> MATQHTQYPDARLSSPIVLDQCDLVTRACGLYSSYSLNPQLRNCKLPKHIYRLKYDVTVTKFLSDVPVATLPIDFIVPILLKALSGNGFCPVEPRCQQFLDEIIKYTMQDALFLKYYLKNVGAQEDCVDDHFQEKILSSIQGNEFLHQMFFWYDLAILTRRGRLNRGNSRSTWFVHDDLIDILGYGDYVFWKIPISLLPLNTQGIPHAAMDWYQTSVFKEAVQGHTHIVSVSTADVLIMCKDLITCRFNTTLISKIAEVEDPVCSDYPNFKIVSMLYQSGDYLLSILGSDGYKIIKFLEPLCLAKIQLCSKYTERKGRFLTQMHLAVNHTLEEITEIRALKPSQAHKIREFHRTLIRLEMTPQQLCELFSIQKHWGHPVLHSETAIQKVKKHATVLKALRPIVIFETYCVFKYSIAKHYFDSQGSWYSVTSDRNLTPGLNSYIKRNQFPPLPMIKELLWEFYHLDHPPLFSTKIISDLSIFIKDRATAVERTCWDAVFEPNVLGYNPPHKFSTKRVPEQFLEQENFSIENVLSYAQKLEYLLPQYRNFSFSLKEKELNVGRTFGKLPYPTRNVQTLCEALLADGLAKAFPSNMMVVTEREQKESLLHQASWHHTSDDFGEHATVRGSSFVTDLEKYNLAFRYEFTAPFIEYCNRCYGVKNVFNWMHYTIPQCYMHVSDYYNPPHNLTLENRNNPPEGPSSYRGHMGGIEGLQQKLWTSISCAQISLVEIKTGFKLRSAVMGDNQCITVLSVFPLETDADEQEQSAEDNAARVAASLAKVTSACGIFLKPDETFVHSGFIYFGKKQYLNGVQLPQSLKTATRMAPLSDAIFDDLQGTLASIGTAFERSISETRHIFPCRIT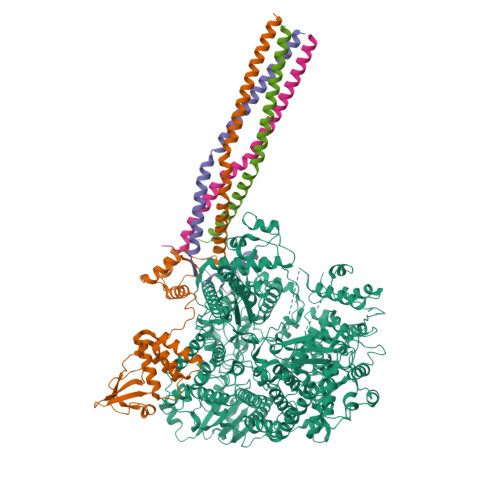AAFHTFFSVRILQYHHLGFNKGFDLGQLTLGKPLDFGTISLALAVPQVLGGLSFLNPEKCFYRNLGDPVTSGLFQLKTYLRMIEMDDLFLPLIAKNPGNCTAIDFVLNPSGLNVPGSQDLTSFLRQIVRRTITLSAKNKLINTLFHASADFEDEMVCKWLLSSTPVMSRFAADIFSRTPSGKRLQILGYLEGTRTLLASKIINNNTETPVLDRLRKITLQRWSLWFSYLDHCDNILAEALTQITCTVDLAQILREYSWAHILEGRPLIGATLPCMIEQFKVVWLKPYEQCPQCSNAKQPGGKPFVSVAVKKHIVSAWPNASRISWTIGDGIPYIGSRTEDKIGQPAIKPKCPSAALREAIELASRLTWVTQGSSNSDLLIKPFLEARVNLSVQEILQMTPSHYSGNIVHRYNDQYSPHSFMANRMSNSATRLIVSTNTLGEFSGGGQSARDSNIIFQNVINYAVALFDIKFRNTEATDIQYNRAHLHLTKCCTREVPAQYLTYTSTLDLDLTRYRENELIYDNNPLKGGLNCNISFDNPFFQGKQLNIIEDDLIRLPHLSGWELAKTIMQSIISDSNNSSTDPISSGETRSFTTHFLTYPKIGLLYSFGAFVSYYLGNTILRTKKLTLDNFLYYLTTQIHNLPHRSLRILKPTFKHASVMSRLMSIDPHFSIYIGGAAGDRGLSDAARLFLRTSISSFLTFVKEWIINRGTIVPLWIVYPLEGQNPTPVNNFLHQIVELLVHDSSRHQAFKTTINDHVHPHDNLVYTCKSTASNFFHASLAYWRSRHRNSNRKDLTRNSSTGSSTNNSDGHIKRSQEQTTRDPHDGTERSLVLQMSHEIKRTTIPQENTHQGPSFQSFLSDSACGTANPKLNFDRSRHNVKSQDHNSASKREGHQIISHRLVLPFFTLSQGTRQLTSSNESQTQDEISKYLRQLRSVIDTTVYCRFTGIVSSMHYKLDEVLWEIENFKSAVTLAEGEGAGALLLIQKYQVKTLFFNTLATESSIESEIVSGMTTPRMLLPVMSKFHNDQIEIILNNSASQITDITNPTWFKDQRARLPRQVEVITMDAETTENINRSKLYEAVHKLILHHVDPSVLKAVVLKVFLSDTEGMLWLNDNLAPFFATGYLIKPITSSARSSEWYLCLTNFLSTTRKMPHQNHLSCKQVILTALQLQIQRSPYWLSHLTQYADCDLHLSYIRLGFPSLEKVLYHRYNLVDSKRGPLVSVTQHLAHLRAEIRELTNDYNQQRQSRTQTYHFIRTAKGRITKLVNDYLKFFLIVQALKHNGTWQAEFKKLPELISVCNRFYHIRDCNCEERFLVQTLYLHRMQDSEVKLIERLTGLLSLFPDGLYRFD;>MTTRTKGRGHTVATTQNDRMPGPELSGWISEQLMTGRIPVNDIFCDIENNPGLCYASQMQQTKPNPKMRNSQTQTDPICNHSFEEVVQTLASLATVVQQQTIASESLEQRITSLENGLKPVYDMAKTISSLNRVCAEMVAKYDLLVMTTGRATATAAATEAYWAEHGQPPPGPSLYEESAIRGKIESRDETVPQSVREAFNNLDSTTSLTEENFGKPDISAKDLRNIMYDHLPGFGTAFHQLVQVICKLGKDSNSLDIIHAEFQASLAEGDSPQCALIQITKRVPIFQDAAPPVIHIRSRGDIPRACQKSLRPVPPSPKIDRGWVCVFQLQDGKTLGLKI[4x]> MLHRSCVLVDSFKEHYHRVHLPRRLALQRYIKR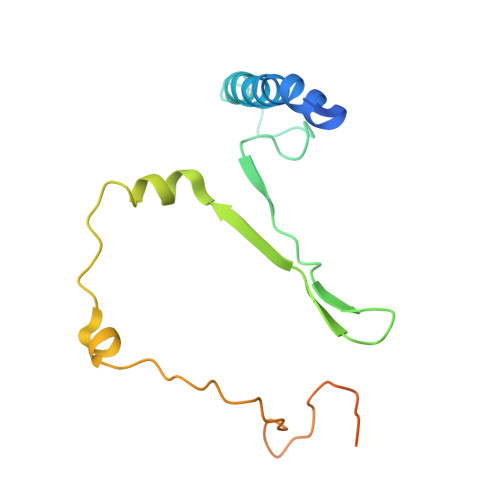EEARLSRHKGKAVAAAAAAGVQPGEVAYKYNRWWVSNDHEFVHQFAFVEDPDVTREKRNTLPLVTKENIWKEPQQTFFLPFAPFVRVVDYAKDPDTKFLKPVNIPRWKDYMQRTKPIVPRTWY> ESTEFEKNQKRYQDLISTFPHEKGWRPKEPLIEYGGYWWLPSLLEGCIHAQEFFQARPSDFLVCSYPKTGTTWLKALTFAIANRSRFDDSSNPLLKRNPHEFVPYIEIDFPFFPEVDVLKDKGNTLFSTHIPYELLPDSVVKSGCKMVYIWREPKDTFISMWTFLHKERTELGPVSNLEESFDMFCRGLSGYGPYLNHILAYWKAYQENPDRILFLKYETMR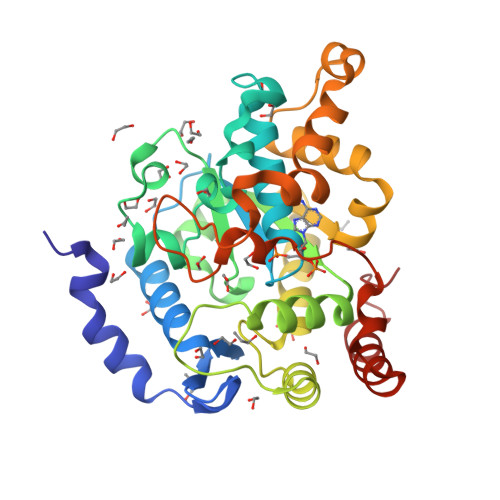ADPLPYVKSLAEFMGHGFTAEEEEKGVVEKVVNLCSFETLKNLEANKGEKDREDRPGVYANSAYFRKGKVGDWSNYLTPEMAARIDGLMEEKFKGTGLLE>MDKSESTSAGRNRRRRPRRGSRSAPSSADANFRVLSQQLSRLNKTLAAGRPTINHPTFVGSERCRPGYTFTSITLKPPKIDRGSYYGKRLLLPDSVTEYDKKLVSRLQIRVNPLPKFDSTVWVTVRKVPASSDLSVAAISAMF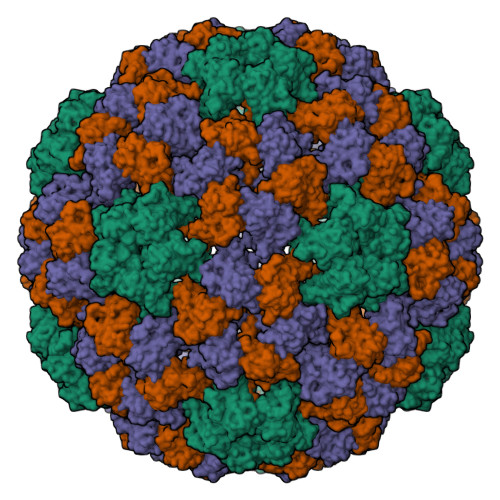ADGASPVLVYQYAASGVQANNKLLYDLSAMRADIGDMRKYAVLVYSKDDALETDELVLHVDIEHQRIPTSGVLPV[3x]> MRIGFNFTLGETLPLVRQLAQEGAIDYCELLIDNFMQVPPQELAEAFDVPVGFHIMFSRFIESDEEQLRDFAARLRPYIEALRPLYVSDHIAYFSHQGRALYHLGEIDYAADYERVRARAALWQSLLGQTIHFENYPSIVDGGHAAPAFFQRLARDTGAGV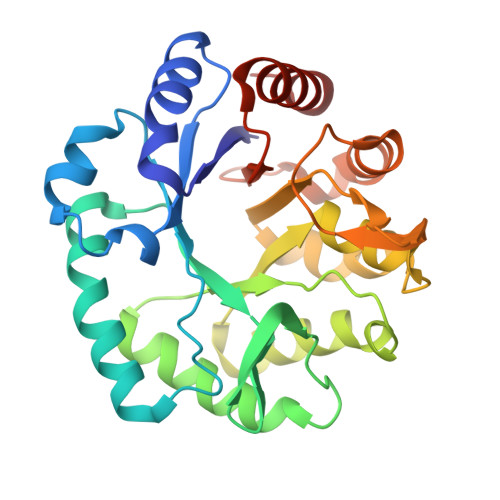LFDVSNAVCAWRNDGPEVAAWRGVMAGASHFHVGGYAGAFIDEGVTVDTHDRALAQDTLDSLRRHRDVLDKPGATITYERDENIDIDGVRADLLALRAIFPRG>MAHHHHHHMFDTSPQLDCAGRILRLDRARVMGIVNVTPDSFSDGGAHDTTEAAVAHGLKLVEEGADLLDIGGESTRPGAAPVSVEEELRRVIPVIEQLAARTRVPISIDTFKPEVMRAAVAAGAGMINDIYGLRQEGALDAAA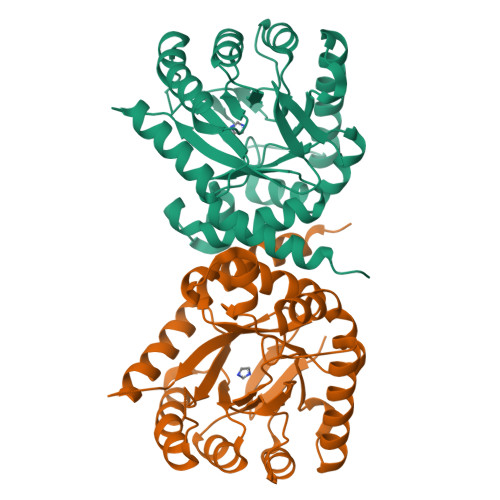ATGVPVVLMHMQGEPGHMQADPHYDDVVAEVHGFLVQRLFAAEMAGFAKKNLLIDLGFGFGKTTAHNMTLLARSERFLELGVPMLAGLSRKRSLGELTGRDTPSERVAASVAAHLIAVQRGARIVRVHDVAATVDALKIWQAVEAVPTPRADATPTIRWPDED[2x]Nicotinamide 2-fluoro-adenine dinucleotide | C21 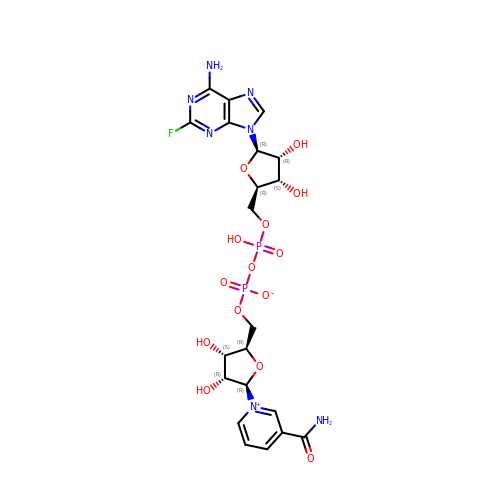H26 F N7 O14 P2 | JDJGJQAJEVFTBI-NAJQWHGHSA-N N-ethyl-6-methoxy-N'-(1-methylethyl)-1,3,5-triazine-2,4-diamine 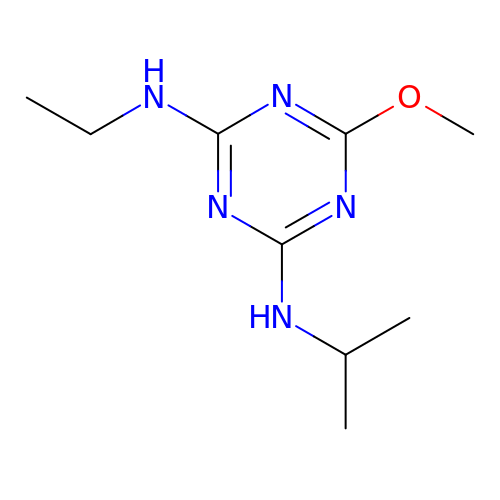| C9 H17 N5 O | PXWUKZGIHQRDHL-UHFFFAOYSA-N> PAARDLKVVTKRGSADGCTDWSVDIKKYQVLVGEPVRIKCALFYGYIRTNYSLAQSA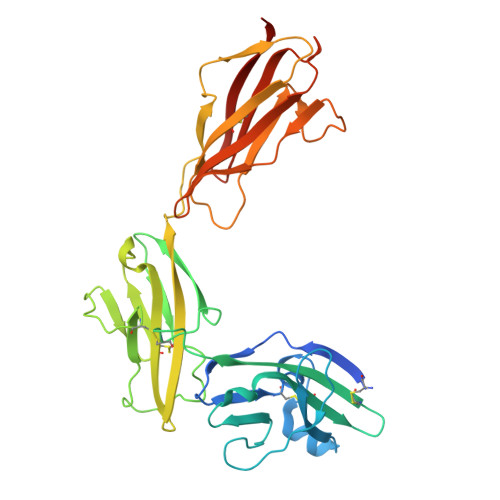GLSLMWYKSSGPGDFEEPIAFDGSRMSKEEDSIWFRPTLLQDSGLYACVIRNSTYCMKVSISLTVGENDTGLCYNSKMKYFEKAELSKSKEISCRDIEDFLLPTREPEILWYKECRTKAWRPSIVFKRDTLLIKEVKEDDIGNYTCELKYGGFVVRRTTELTVTAPLTDKPPKLLYPMESKLTVQETQLGGSANLTCRAFFGYSGDVSPLIYWMKGEKFIEDLDENRVWESDIRILKEHLGEQEVSISLIVDSVEEGDLGNYSCYVENGNGRRHASVLLHKRKHHHHHH The staphylococcal phage lysin LysGH15 demonstrates great potential against methicillin-resistant Staphylococcus aureus (MRSA). Lysin (also known as endolysin) is a cell wall hydrolase that is synthesized at the end of the phage lytic life cycle and is involved in cell lysis and the release of progeny particles from host cells. LysGH15 shares very high sequence identity with other lysins of class III staphylococcal phages, such as LysK, phi11, and MV-L. Moreover, these lysins possess a modular structure containing an N-terminal CHAP domain (cysteine, histidine-dependent amidohydrolases/peptidases), a central amidase-2 domain (N-acetylmuramoyl-L-alanine amidase), and a C-terminal SH3b domain (the SH3 bacterial binding domain, which typically contains 60–70 residues and is homologous to eukaryotic SH3 proteins). To elucidate the molecular mechanism, we determined the structures of three individual LysGH15 domains using X-ray crystallography or nuclear magnetic resonance (NMR).

The CHAP domain crystallizes in the P6222 space group with two molecules in the asymmetric unit (ASU). The quality of the electron density permits the unambiguous modeling of residues 1–164. The two molecules form a dimer that is mediated by hydrogen bonding interactions at the central interface by one molecule of Bis-Tris-propane that was present in the crystallization reservoir solution. However, a Bis-Tris-propane molecule does not mediate homodimer formation of the CHAP domain in solution and cannot affect the activity of the CHAP domain. The crystal structure of the CHAP domain unexpectedly reveals a calcium-binding site near the Cys-His-Glu-Asn quartet active site (the active site that consists of cysteine, histidine, glutamic acid, and asparagine typically found in members of the CHAP family), and site-directed mutagenesis further confirms that both the calcium ion binding site and the conserved Cys-His-Glu-Asn quartet are required for the lytic activity of the LysGH15 CHAP domain. Although the calcium-binding loop of the LysGH15 CHAP domain is 12 residues in length (the coordination residues lie at positions 1, 3, 5, 7, and 12), the secondary structure elements surrounding the calcium-binding site of the CHAP domain only contain one helix, which is consistent with an “EF-hand-like” motif. Note that D45, D47, and D56 coordinate the calcium ion via their side chains, whereas Y49 and H51 coordinate the calcium ion via their main chains. In the center of the groove, C54, H117, E134, and N136 form the Cys-His-Glu-Asn quartet. However, in light of its location near the active site groove and its significant influence on the lytic activity of the protein, there are two potential functions for this calcium ion: (i) it participates in the catalytic activity as part of the reaction; or (ii) it positions the key residues, particularly C54, to form the appropriate conformation.

>[2x]SNAMAKTQAEINKRLDAYAKGTVDSPYRIKKATSYDPSFGVMEAGAIDADGYYHAQCQDLITDYVLWLTDNKVRTWGNAKDQIKQSYGTGFKIHENKPSTVPKKGWIAVFTSGSYQQWGHIGIVYDGGNTSTFTILEQNWNGYANKKPTKRVDNYYGLTHFIEIPVKA>GHMVDTSGVKIHPAVDNGIKPAQPGFAGGTLHCKCSTNPVRVAVRAQTAHNHVCGCTKCWKPEGAIFSQVAVVGRDALEVLEGAEKLEIVNAEAPIQRHRCRDCGVHMYGRIENRDHPFYGLDFVHTELSDEDGW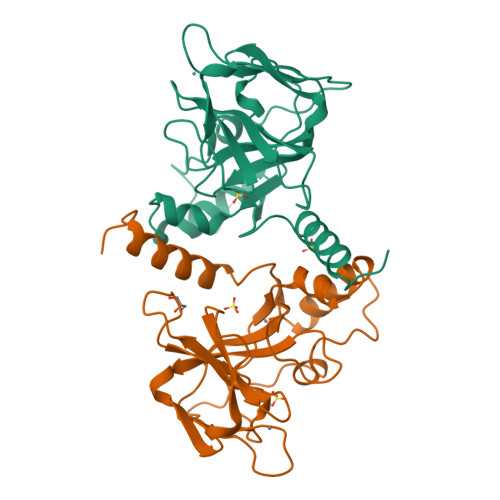SAPEFAAFVSSIIESGVDPSRMEAIRARLRELGLEPYDALSPPLMDAIATHIAKRSGALAA[4x]> HMRKKIFKPEELRQALMPTLEALYRQDPESLPFRQPVDPQLLGIPDYFDIVKNPMDLSTIKRKLDTGQYQEPWQYVDDVWLMFNNAWLYNRKTSRVYKFCSKLAEVFE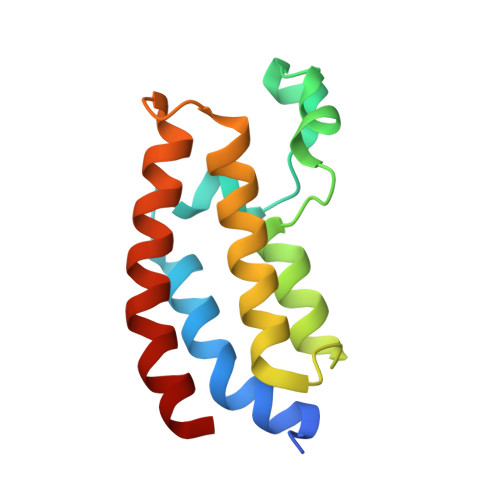QEIDPVMQSL>MENTVLNLDSDVIHACEAIFQPIRLVYTHAQTPDVSGVSMLEKIQQILPQIAKNAESAEQLRRVPDENIKLLKEIGLHRAFQPKVYGGLEMSLPDFANCIVTLAGACAGTAWAFSLLCTHSHQIAMFSKQLQDEIWLKDPDATASSSIAPFGKVEEVEGGIILNGDYGWSSGCDHAEYAIVGFNRFDADGNKIYSFGVIPRSDYEIVDNWYAQAIKSSGSKMLKLVNVFIPEYRISKAKDMMEGKSAGFGLYPDSKIFYTPYRPYFASGFSAVSLGIAERMIEAFKEKQRNRVRAYTGANVGLATPALMRIAESTHQVAAARALLEKTWEDHRIHGLNHQYPNKETLAFWRTN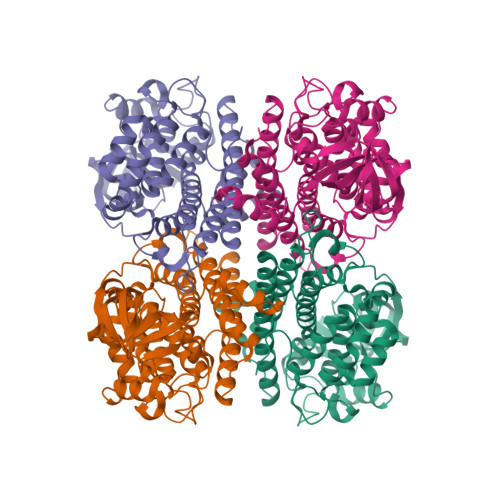QAYAVKMCIEAVDRLMAAAGATSFMDNSELQRLFRDAHMTGAHAYTDYDVCAQILGRELMGMEPDPTMV[4x]>SRCTHLENRDFVTGTQGTTRVTLVLELGGCVTITAEGKPSMDVWLDAIYQENPAKTREYCLHAKLSDTKVAARCPTMGPATLAEEHQGGTVCKRDQSDRGWGNHCGLFGKGSIVACVKAACEAKKKATGHVYDANKIVYTVKVEPHTGDYVAANETHSGRKTASFTISSEKTILTMGEYGDVSLLCRVASGVDLAQTVILELDKTVEHLPTAWQVHRDWFNDLALPWKHEGAQNWNNAERLVEFGAPHAVKMDVYNLGDQTGVLLKALAGVPVAHIEGTKYHLKSGHVTCEVGLEKLKMKGLTYTMCDKTKFTWKRAPTDSGHDTVVMEVTFSGTKPCRIPVRAVAHGSPDVNVAMLITPNPTIENNGGGFIEMQLPPGDNIIYVGELSH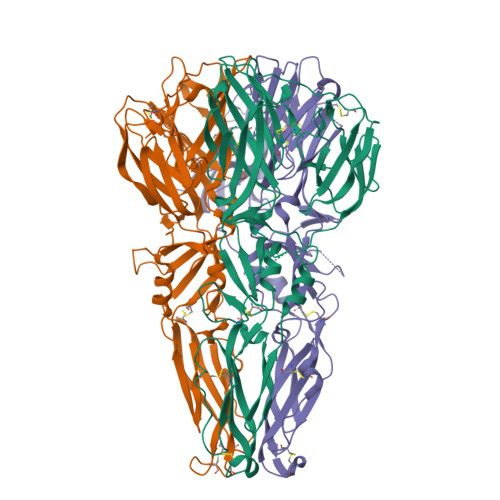QWFQKGSSIGR[6x]> GSHMKFTVEREHLLKPLQQVSGPLGGRPTLPILGNLLLQVADGTLSLTGTDLEMEMVARVALVQPHEPGATTVPARKFFDICRGLPEGAEIAVQLEGERMLVRSGRSRFSLSTLPAADFPNLDDWQSEVEFTLPQATMKRLIEATQFSMAHQDVRYYLNGMLFETE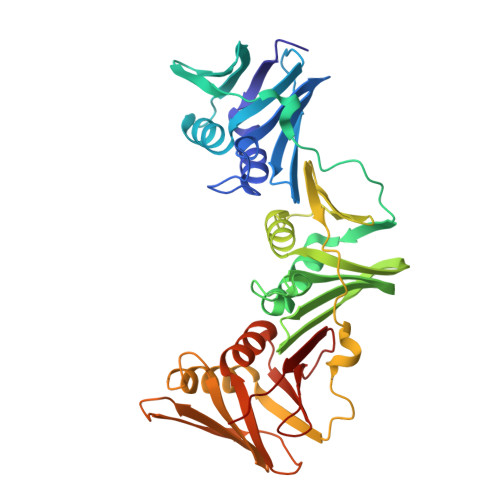GEELRTVATDGHRLAVCSMPIGQSLPSHSVIVPRKGVIELMRMLDGGDNPLRVQIGSNNIRAHVGDFIFTSKLVDGRFPDYRRVLPKNPDKHLEAGCDLLKQAFARAAILSNEKFRGVRLYVSENQLKITANNPEQEEAEEILDVTYSGAEMEIGFNVSYVLDVLNALKCENVRMMLTDSVSSVQIEDAASQSAAYVVMPMRL> VVSFIGSTENDVGPSQGSYSSTHAMDNLPFVYNTGYNIGYQNANVWRIGGGFCVGLDGKVDLPVVGSLDGQSIYGLTEEVGLLIWMGDTNYSRGTAMSGNSWENVF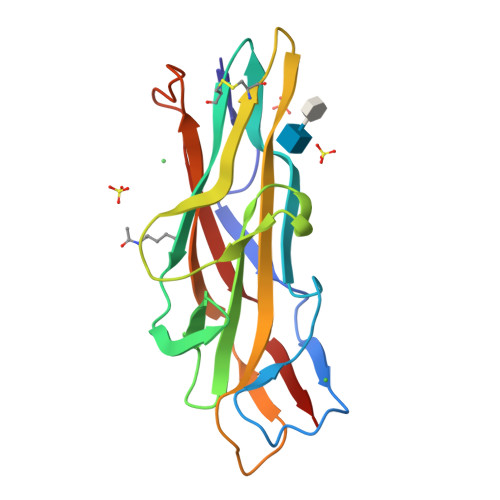SGWCVGNYLSTQGLSVHVRPVILKRNSSAQYSVQKTSIGSIRMRPYNGSSAGSVQTTVNFSLNPFTLNDT> MSQSVSERTRIKSDRYESGVIPYAKMGYWDASYTVKDTDVLALFRITPQPGVDPVEAAAAVAGESSTATWTVVWTDLLTACERYRAKAYRVDPVPNSADVFFAFIAYECDLFEEASLANLTASIIGNVFGFKAVSALRLEDMRIPHSYLXTFQGPAT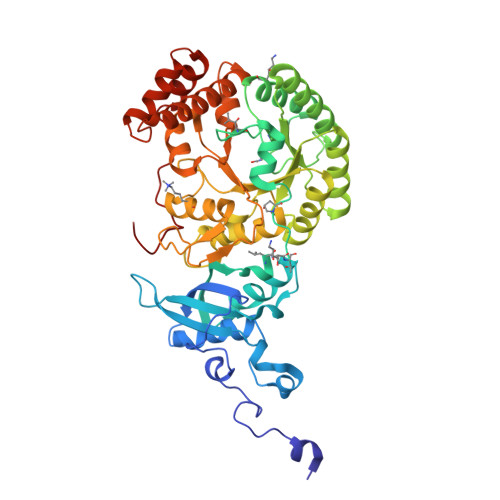GIIVERERLNKYGTPLLGATVKPKLGLSGKNYGRVVYEGLKGGLDFLKDDENINSQPFMRWRERFLNCMEGINRASAATGEVKGSYLNITAATMEEVYKRAEYAKAVGSIVVMIDLVMGYTAIQSIAYWARENDMLLHLHRAGNSTYARQKNHGINFRVICKWMRMSGVDHIHAGTVVGKLEGDPLMIKGFYDILRLTELEVNLPFGIFFEMDWASLRRCMPVASGGIHCGQMHQLIHYLGDDVVLQFGGGTIGHPDGIQAGATANRVALESMVLARNEGVDYFDQQVGPQILRDAAKTCGPLQTALDLWKDISFDYTSTDTADFAE>GPLGSMEDAKNIKKGPAPFYPLEDGTAGEQLHKAMKRYALVPGTIAFTDAHIEVNITYAEYFEMSVRLAEAMKRYGLNTNHRIVVCSENSLQFFMPVLGALFIGVAVAPANDIYNERELLNSMNISQPTVVFVSKKGLQKILNVQKKLPIIQKIIIMDSKTDYQGFQSMYTFVTSHLPPGFNEYDFVPESFDRDKTIALIMNSSGSTGLPKGVALPHRTACVRFSHARDPIFGNQIIPDTAILSVVPFHHGFGMFTTLGYLICGFRVVLMYR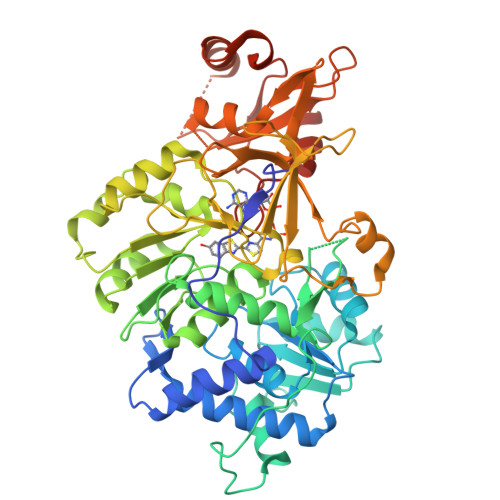FEEELFLRSLQDYKIQSALLVPTLFSFFAKSTLIDKYDLSNLHEIASGGAPLSKEVGEAVAKRFHLPGIRQGYGLTETTSAILITPEGDDKPGAVGKVVPFFEAKVVDLDTGKTLGVNQRGELCVRGPMIMSGYVNNPEATNALIDKDGWLHSGDIAYWDEDEHFFIVDRLKSLIKYKGYQVAPAELESILLQHPNIFDAGVAGLPDDDAGELPAAVVVLEHGKTMTEKEIVDYVASQVTTAKKLRGGVVFVDEVPKGLTGKLDARKIREILIKAKKGGKSKL[2x]> GVALGATRVIYPAGQKQVQLAVTNNDENSTYLIQSWVENADGVKDGRFIVTPPLFAMKGKKENTLRILDATNNQLPQDRESLFWMNVKAIPSMDKSKLTENTLQLAIISRIKLYYRPAKLALPPDQAAEKLRFRRSANSLTLINPTPYYLTVTELNAGTRVLENALVPPMGESTVKLPSDAGSNITYRTINDYGALTPKMTGVMEHHHHHH;> DLYFNPRFLADDPQAVADLSRFENGQELPPGTYRVDIYLNNGYMATRDVTFNTGDSEQGIVPCLTRAQLASMGLNTASVAGMNLLADDACVPLTTMVQDATAHLDVGQQRLNLTIPQAFMSNRARGYIPPELWDPGINAGLLNYNFSGNSVQNRIGGNSHYAYLNLQSGLNIGAWRLRDNTTWSYNSSDRSSGSKNKWQHINTWLERDIIPLRSRLTLGDGYTQGDIFDGINFRGAQLASDDNMLPDSQRGFAPVIHGIARGTAQVTIKQNGYDIYNSTVPPGPFTINDIYAAGNSGDLQVTIKEADGSTQIFTVPYSSVPLLQREGHTRYSITAGEYRSGNAQQEKPRFFQSTLLHGLPAGWTIYGGTQLADRYRAFNFGIGKNMGALGALSVDMTQANSTLPDDSQHDGQSVRFLYNKSLNESGTNIQLVGYRYSTSGYFNFADTTYSRMNGYNIETQDGVIQVKPKFTDYYNLAYNKRGKLQLTVTQQLGRTSTLYLSGSHQTYWGTSNVDEQFQAGLNTAFEDINWTLSYSLTKNAWQKGRDQMLALNVNIPFSHWLRSDSKSQWRHASASYSMSHDLNGRMTNLAGVYGTLLEDNNLSYSVQTGYAGGGDGNSGSTGYATLNYRGGYGNANIGYSHSDDIKQLYYGVSGGVLAHANGVTLGQPLNDTVVLVKAPGAKDAKVENQTGVRTDWRGYAVLPYATEYRENRVALDTNTLADNVDLDNAVANVVPTRGAIVRAEFKARVGIKLLMTLTHNNKPLPFGAMVTSESSQSSGIVADNGQVYLSGMPLAGKVQVKWGEEENAHCVANYQLPPESQQQLLTQLSAECR;> ADSTITIRGYVRDNGCSVAAESTNFTVDLMENAAKQFNNIGATTPVVPFRILLSPCGNAVSAVKVGFTGVADSHNANLLALENTVSAASGLGIQLLNEQQNQIPLNAPSSALSWTTLTPGKPNTLNFYARLMATQVPVTAGHINATATFTLEYQ;> FACKTANGTAIPIGGGSANVYVNLAPVVNVGQNLVVDLSTQIFCHNDYPETITDYVTLQRGSAYGGVLSNFSGTVKYSGSSYPFPTTSETPRVVYNSRTDKPWPVALYLTPVSSAGGVAIKAGSLIAVLILRQTNNYNSDDFQFVWNIYANNDVVVPTGGCDVSARDVTVTLPDYPGSVPIPLTVYCAKSQNLGYYLSGTTADAGNSIFTNTASFSPAQGVGVQLTRNGTIIPANNTVSLGAVGTSAVSLGLTANYARTGGQVTAGNVQSIIGVTFVYQ

Type 1 pili expressed by uropathogenic Escherichia coli (UPEC) are tipped by an adhesin, FimH, that binds mannosylated glycoproteins, including those on the surface of bladder epithelial cells to facilitate attachment to and invasion of bladder superficial facet cells. Assembly of type 1 pili is facilitated by the FimC periplasmic chaperone and FimD outer-membrane (OM) usher in an ATP-independent manner. At the usher, the Nte on an incoming subunit displaces the chaperone’s G1 β-strand and completes the subunit fold of the preceding subunit in a canonical (antiparallel) and energetically favored manner, termed donor-strand exchange (DSE). X-ray and cryoelectron microscopy (cryo-EM) structures of FimD–FimCFGH demonstrate large coordinated movements of the five usher domains involved in catalyzing DSE interactions between neighboring subunits and extrusion of the growing fiber. These structures also show that the two-domain adhesin FimH, which consists of the lectin (FimHL) and pilin (FimHP) domains, adopts an elongated (“relaxed”) or bent (“tense”) configuration prior to and after secretion to the extracellular surface, respectively.

Here, we report the cryo-EM structure of a quaternary complex FimD–FimCFH, in which the FimH adhesin is in a previously unseen location within the pore of the FimD usher during transport. The FimD–FimCH structure had a reported overall resolution of ~3.5 Å and was essentially identical to that published previously, while the FimD–FimCFH structure, at ~4.0 Å resolution, revealed a previously unreported assembly intermediate enabled by DSE between FimH and FimF. Unlike the previously determined initiation and elongation structures, this complex reveals FimH positioned halfway in the usher pore. Remarkably, during this stage in secretion, FimH adopts a third “relaxed-stretched” conformation involving both an elongation and rotation between its pilin and lectin domains. Thus, we termed this conformation “relaxed-stretched. This conformation is adopted by FimH as it spans the entire OM while retaining contact with both the periplasmic and extracellular spaces. In this model, FimH is linked to FimF through DSE between FimH and FimF. The chaperone–subunit complex FimC–FimF makes contacts with both the CTDs and N-terminal tail of the usher FimD. With the engagement of only two pilin subunits (FimH and FimF), the FimHP domain is partially inserted into the TD pore as FimF, having undergone DSE with FimHP, remains bound to the chaperone FimC and held by the usher NTD and CTDs in the periplasmic space. In contrast, the pilin domain FimHP undergoes substantial reorientation (a rotation of 84°) to be compatible with its residency in the TD pore. During secretion, FimH is obligated to adopt a third, “relaxed-stretched” conformation, in which the two domains are maximally apart from each other.>[4x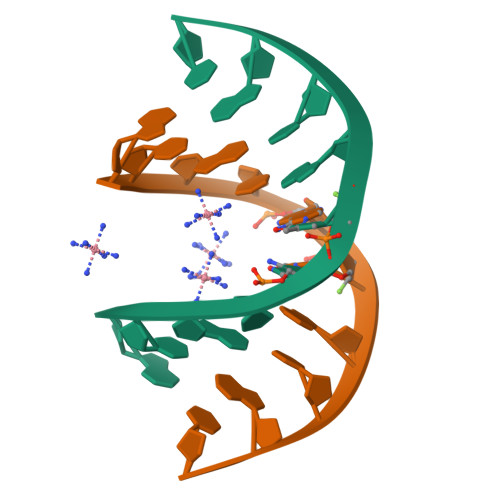]GCGTATACGC>MQATLIKPTIFTHQPILEKLFKSQSMTQEESHQLFAAIVRGELEDSQLAAALISMKMRGERPEEIAGAASALLADAQPFPRPDYDFADIVGTGGDGTNSINISTASAFVAASCGAKVAKHGNRSVCQPLAGSCDLLQAFGIRLDMSAEDSRQALDDLNVCFLFAPQYHTGFRHAMPVRQQLKTRTIFNVLGPLINPARPPKALIGVYSPELVLPIAQALKVLGYKNAAVVHGGGMDEVAIHTPTQVAELNNGEIESYQLSPQDFGLQSYSLNALQGGTPEENRDILARLLQGKGDAAHARQVAANVALLLKLFGQDNLRHNAQLAL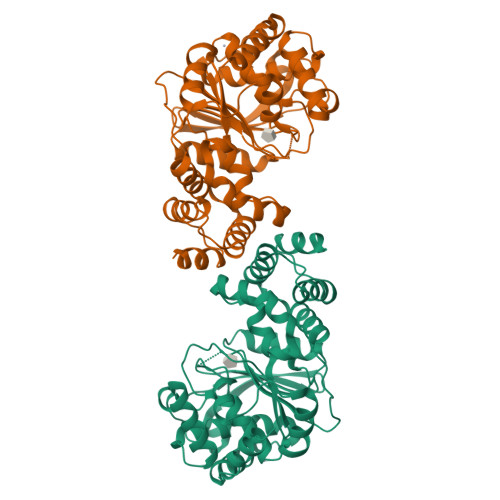ETIRSGTAFERVTALAARG[2x]> VEWTDKERSIISDIFSHMDYDDIGPKALSRCLVVYPWTQRYFSGFGNLYNAEGIMSNANVAAHGIKVLHGLDRGMKNMDNIADAYTDLSTLHSEKLHVDPDNFKLLSDCITIVLAAKMGHAFTAETQGAFQKFLAAVVSALG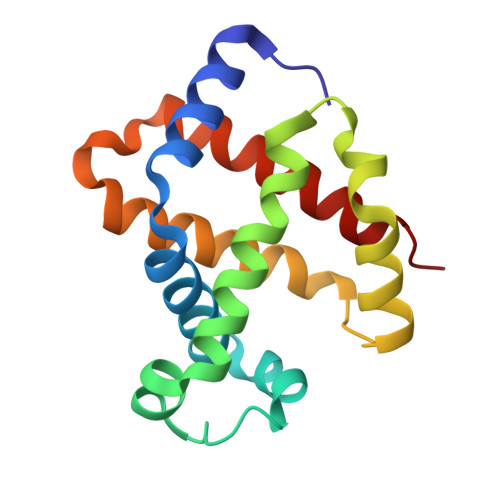KQYH To investigate the correlation between mechanical properties and functional efficiency in proteins, we selected neuroglobin (Ngb), a hexacoordinated heme protein, which is expressed in the neurons of vertebrates and is involved in neuroprotection in hypoxic conditions and protects brain from stroke. Ngb folds like all globins with a bundle of eight helices termed A to H, and a heme hexacoordinated in both ferric and ferrous forms by the imidazole side chain of the distal and proximal histidines (His 64 and His 96 respectively). The structures of human and murine Ngb present a large internal cavity behind the heme, that is connected to the surface through a tunnel, forming a pathway toward the heme for gaseous ligands (O2, CO, NO). Like many recently discovered globins, Ngb is characterized by endogenous heme iron hexacoordination in the absence of external ligands.

Residue Val 101, located in the FG loop, points toward the heme on the proximal heme side. Its substitution by a bulkier Phe residue was designed to decrease the volume of the internal cavity. The crystal structure of this mutant was not previously known, consequently the reference structure V101F AP, though to describe the effects of the mutation only, was determined. The mutation of Val 101 to a Phe residue leads to a shift of the beginning of helix G (Leu 103 – Ser 107) toward the bulk by almost 1 Å (on Cα chain), while helix F is mostly unaffected. In more detail, the side chain of Phe 101 pushes by 1 Å the side chain of Phe 106 toward the position it occupies when the heme has slid into the cavity in the CO-Ngb structure. In turn, the side chain of Phe 106 displaces the side chain of Leu 103 to the position it occupied in the CO-Ngb structure. The positions of the heme, the proximal and the distal histidines are unaffected by the mutation. Contrary to expectations, the volume of the internal cavity increases by almost 5% upon the Val 101 to Phe mutation, due to the shift of helix G away from the heme. Moreover, helix G in the V101F mutant shifts toward the bulk exactly in the same position it occupies in the CO-Ngb structure, while helix F stays as it is in the hexacoordinate structure. Unexpectedly, the introduction of a Phe at position 101 located in FG loop induces the displacement of Phe 106 in the position observed in the CO-Ngb structure, i.e. when gaseous ligand is bound and the heme sliding accomplished. This may explain why V101F mutant showed unaffected CO affinity.

> RPESELIRQSWRVVSRSPLEHGTVLFARLFALEPSLLPLFQYNGRQFSSPEDSLSSPEFLDHIRKVMLVIDAAVTNVEDLSSLEEYLTSLGRKHRAVGFRLSSFSTVGESLLYMLEKSLGPDFTPATRTAWSRLYGAVVQAMSRGWDG>[4x]SIVIASAARTAVGSFNGAFANTPAHELGATVISAVLERAGVAAGEVNEVILGQVLPAGEGQNPARQAAMKAGVPQEATAWGMNQLCGSGLRAVALGMQQIATGDASIIVAGGMESMSMAPHCAHLRGGVKMGDFKMIDTMIKDGLTDAFYGYHMGTTAENVAKQWQLSRDEQDAFAVASQNKAEAAQKDGRFKDEIVPFIVKGRKGDITVDADEYIRHGATLDSM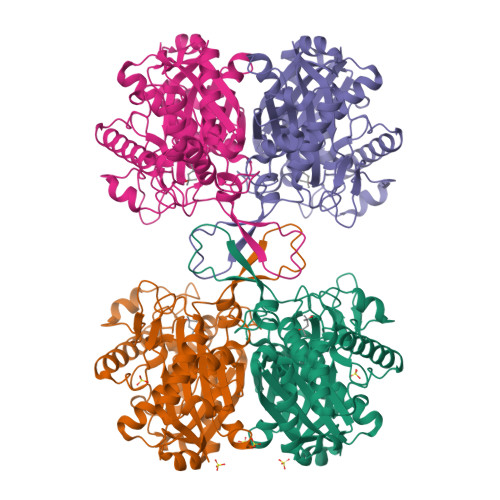AKLRPAFDKEGTVTAGNASGLNDGAAAALLMSEAEASRRGIQPLGRIVSWATVGVDPKVMGTGPIPASRKALERAGWKIGDLDLVEANEAFAAQACAVNKDLGWDPSIVNVNGGAIAIGHPIGASGARILNTLLFEMKRRGARKGLATLCIGGGMGVAMCIESL The gene encoding for ChiP is found in most marine members of the Vibrionaceae, emphasizing the general importance of this OM diffusion channel for chitin utilization. The addition of micromolar concentrations of chitooligosaccharides such as chitohexaose (GlcNAc6) causes a complete block of ionic current, demonstrating tight binding. Here, we report X-ray crystal structures of VhChiP in the absence and presence of chitooligosaccharides.

Subsequently we cloned VhChiP without a signal sequence and with a C-terminal His6-tag into pET28a to express the protein into inclusion bodies (IBs) and avoid toxicity issues. VhChiP from IBs was folded in vitro from 8 M urea and purified as the native protein. Well-diffracting crystals (~ 2 Å resolution) in space group P21 were obtained and a SAD data set was collected at the absorption edge of Selenium. In vitro-folded VhChiP forms a trimeric assembly of oval β-barrels, each consisting of 16 strands, like the general diffusion porins OmpF/C from E. coli. Unlike OmpF/C however, the N-terminus of VhChiP does not form an intramolecular salt bridge with the C-terminal carboxyl group. Instead, the first N-terminal 17 amino acids of VhChiP are not part of the barrel and extend into the periplasm where they form a trimerization motif like that observed in the phosphate transporter OprP from Pseudomonas aeruginosa. The first nine amino acids of the N-terminus are disordered and not visible in the electron density. Thus, five out of the first six residues of the N-terminus make polar interactions with the pore of the protein, suggesting that the plug is stably inserted in the pore. It should be noted that for in vitro-folded VhChiP, two residues (MG) were added to the N-terminus of the mature protein for inclusion body expression, and it is possible that the presence of those additional residues has destabilized the plug sufficiently for it be outside the pore. The N-terminal ten residues of in vitro-folded VhChiP are highly flexible and do not insert into the pore. Consistent with the experiments, the in vitro-folded trimeric channel shows a theoretical conductance value of 2.13 ± 0.15 nS, only slightly higher than the experimental value of 1.8 nS measured at lower voltages.

>MGDGANSDAAKEYLTKDSFSYEVYGIIAMQAAYRDYDSGDAKQDDNLGGMQLNNESRIGFRGKKQFANFEPTFIWQIEGGYVDPSFGGEGAGLGERDTFVGFESASWGQVRLGRVLTPMYELVDWPASNPGLGDVYDWGGAIGGAKYQDRQSNTIRWDSPMYADKFSIDAAVGAGDKAGLGAGDDYWGGIAAHYKLGPLQLDAAYEGNRNIEAEGQTWENNTYLVGVQGWFENGISFFAQYKYMEADASNGVNEKQDAMSAGLMYTTGDWQYKLGYAANFDLERDGKTLSNTSDDVVSAQIMYFVDPSAVLYARARMNDFNEGLDGLDDAARWTSGTNGDYNEYSVGVEYYF[6x]>EELPQIEIVQEGDNTTFAKPGDTVTIHYDGKLTNGKEFDSSRKRGKPFTCTVGVGQVIKGWDISLTNNYGKGGANLPKISKGTK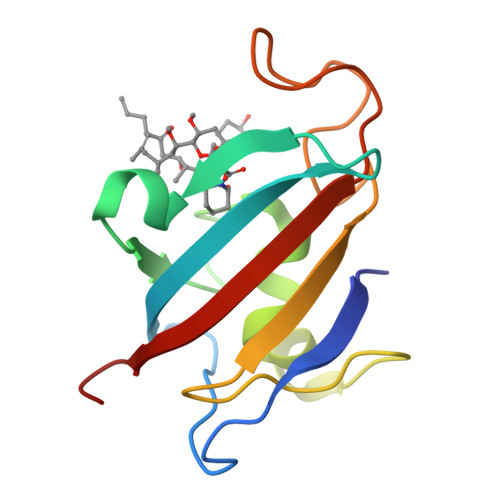AILTIPPNLAYGPRGIPGIIGPNETLVFEVELLGVNGQ[8x]(3S)-3-(4-CHLOROPHENYL)-4-(5,7-DICHLORO-1H-BENZIMIDAZOL-2-YL)BUTANOIC 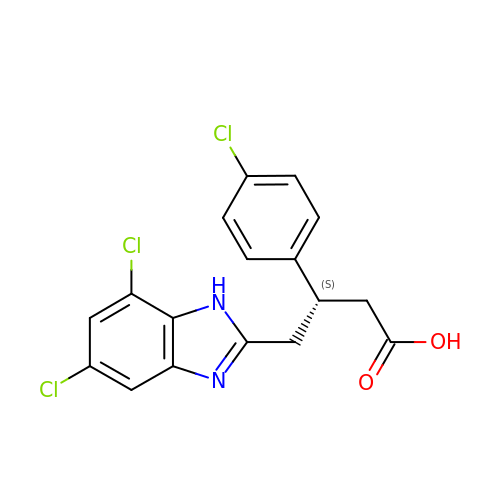ACID | C17 H13 Cl3 N2 O2 | WMLLAHSMFYNLLO-JTQLQIEISA-N> MKEYTLDKAHTDVGFKIKHLQISNVKGNFKDYSAVIDFDPASAEFKKLDVTIKIASVNTENQTRDNHLQQDDFFKAKKYPDMTFTMKKYEKIDNEKGKMTGTLTIAGVSKDIVLDAEIGGVAKGKDGKEKIGFSLNGKIKRSDFKFATSTST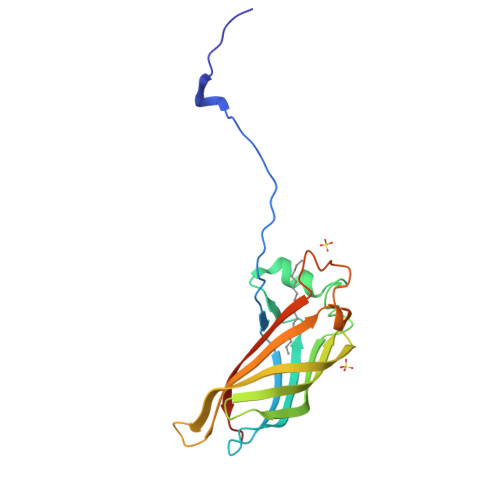ITLSDDINLCIEVEANEKEGGSHHHHHH(4aR,6aR,6aS,6bS,8aS,9R,12aR,14bR)-2,2,6a,6b,9,12a-hexamethyl-10-oxidanylidene-1,3,4,5,6,6a,7,8,8a,9,11,12,13,14b-tetradecahydropicene-4a-carboxylic acid | C29 H44 O3 | 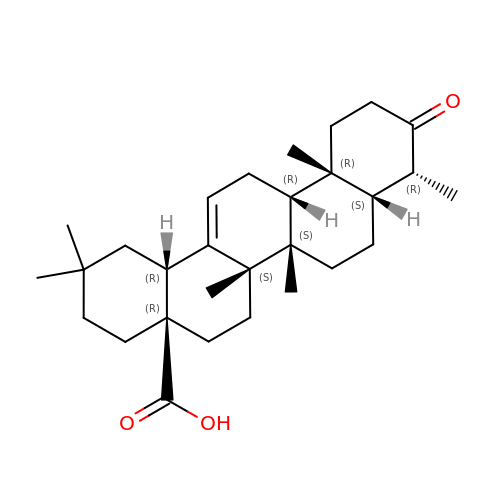USBFNWRNJYBPQP-IQJSWQEESA-N> MTRVVAGDVGTDTPDKAGTADTAKA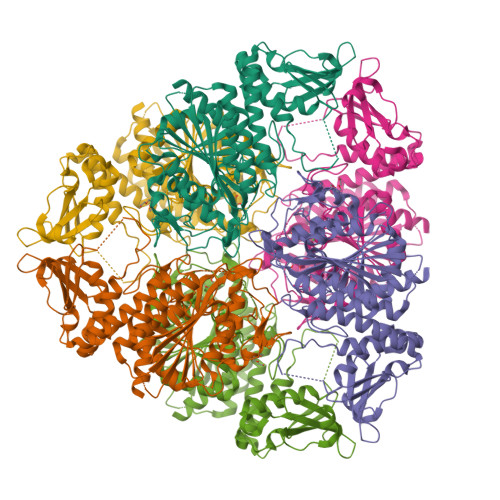ADTADTASRAADVVACGRHTGAAVGAFSRRRGFVARPGQVVAEPSADGRAVVLNVGLGPAGSATAATFRAAAAASVRAVGPARTLRLDLALADGSGVPAAERARAVAEGAVLGLYRYDEYRSARAASPLAEVIVATPERRAVAEGLAAAEATCLARDLVNCPAGTLTPPAFADRIRELAHTAGLDCAVYEGAGLTELGLTGLTAVGRGSAEPPRYVELTYDPPDADPALTVGLVGKGVTFDSGGLSLKPSGERHAMKADMGGAAAVVAALTALPRLGLPLRVRGHLPLAENMPDGGALRVGDVVRHLDGTTTEITHTDNEGRVVLADVLVRASRPGPHRSDLVVDVATLTSAAVHALGTRTGALFTPDDRLAQTVLAASERAGESFCRLPLLAHERRNLRSAVADRVNCSHRHGDTIQAALFLQDFVAAGVPWAHLDIAAPAYNDEGPYAEVPYGGTGFAVRTLIETLRALSEGSPDVP>MGSDKIHHHHHHMKKLTVYLATTNPHKVEEIKMIAPEWMEILPSPEKIEVVEDGETFLENSVKKAVVYGKKLKHPVMADDSGLVIYSLGGFPGVMSARFMEEHSYKEKMRTILKMLEGKDRRAAFVCSATFFDPVENTLISVEDRVEGRIANEIRGTGGFGYDPFFIPDGYDKTFGE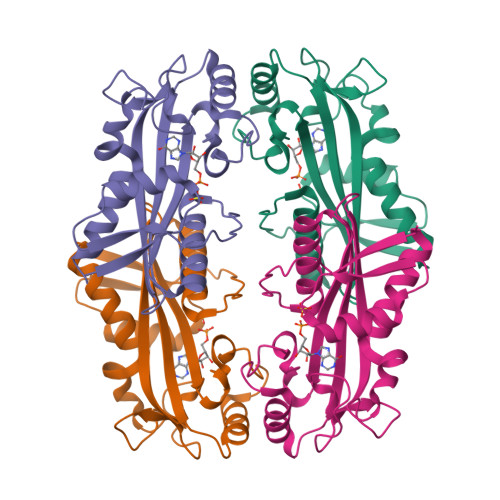IPHLKEKISHRSKAFRKLFSVLEKILESENR[4x]>TKTGYINAAFRSSRNNEAYLFINDKYVLLDYAPGTSNDKVLYGPSFVRDGYKSLAKTIFGTYGIDCSFDTEYNEAFIFYENFCARIDYAPHSDKDKIISGPKKIADMFPFFKGTVFENGIDAAFRSTKGKEVYLFKGDKYARIDYLTNRLVQNKSISDTGFPCLRGTIFEAGMDSAFASHKTNEAYLFKGEYYARINFTPGSTNDIMGGVKKTLDYWPSL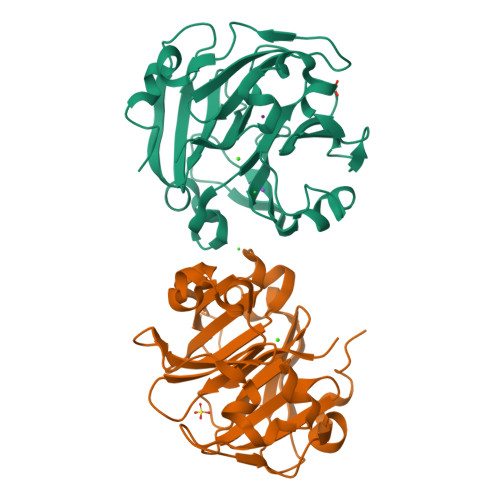RGIIPLE[2x]>[2x]SLHSPGKAFRAALTKENPLQIVGTINANHALLAQRAGYQAIYLSGGGVAAGSLGLPDLGISTLDDVLTDIRRITDVCSLPLLVDADIGFGSSAFNVARTVKSMIKAGAAGLHIEDQVGAKRCGHRPNKAIVSKEEMVDRIRAAVDAKTDPDFVIMARTDAL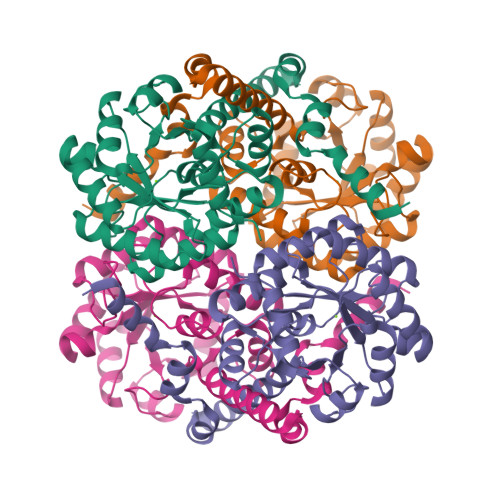AVEGLDAAIERAQAYVEAGAEMLFPEAITELAMYRQFADAVQVPILANITEFGATPLFTTDELRSAHVAMALYPLSAFRAMNRAAEHVYNVLRQEGTQKSVIDTMQTRNELYESINYYQYEEKLDNLFARSQVK GLIC, a prokaryotic ligand-gated ion channel found in Gloeobacter violaceus, served as a model system to comprehend the gating mechanism of eukaryotic ligand-gated channels. The overall architecture of GLIC is similar to the existing structures with each monomer featuring two domains: the ECD, mainly composed of β strands and the TMD, composed of four α helices (M1-M4). In this study, we present cryo-EM structures of GLIC reconstituted in lipid nanodiscs at pH 7.5, 5.5, 4.0, and 2.5. We identified a resting-like state, two putative intermediate states, a putative pre-open state, and an open state.

Two cryo-EM structures of GLIC reconstituted in either soybean polar lipid extract (or asolectin referred to as “aso” onwards) or DOPE:POPS:POPC (2:1:1) at pH 7.5 were obtained with a nominal resolution of 3.4 and 2.9 Å, respectively. Local resolution estimation of these two maps (referred here onwards as GLICaso-pH7.5 and GLICpH7.5) in the apo state shows higher resolution in TMD than ECD. A comparison between GLICaso-pH7.5 and GLICpH7.5 structures shows overlapping secondary structures with minimum conformational differences and a backbone (Cα) RMSD of 0.52 Å. A similar conformation of GLICpH7.5 and GLICaso-pH7.5 confirms the minimal impact of distinct lipid compositions on the GLIC structure in the apo state. Multiple constrictions at the pore of GLICaso-pH7.5 and GLICpH7.5 are observed, with the most significant constrictions at I16´, I9´, and T2´. The highest constriction is observed at I9´ with a radius of ~2.24 Å. However, the radius at I9´ falls below the radius of a hydrated Na+ ion (2.76 Å), reflecting a non-conducting state. Truncated phospholipids (PC in GLICaso-pH7.5 and PE in other structures) were placed in partially resolved non-protein lipid-like densities. In GLICaso-pH7.5, the head group of Lipid 1 is involved in polar interaction with the backbone amide group of M252 located at the M2–M3 loop and this interaction is not observed in GLICpH7.5 and GLICpH5.5. Therefore, our GLICpH7.5 and GLICaso-pH7.5 represent a state closer to the resting conformation.

>[5x]VSPPPPIADEPLTVNTGIYLIECYSLDDKAETFKVNAFLSLSWKDRRLAFDPVRSGVRVKTYEPEAIWIPEIRFVNVENARDADVVDISVSPDGTVQYLERFSARVLSPLDFRRYPFDSQTLHIYLIVRSVDTRNIVLAVDLEKVGKNDDVFLTGWDIESFTAVVKPANFALEDRLESKLDYQLRISRQYFSYIPNIILPMLFILFISWTAFWSTSYEANVTLVVSTLIAHIAFNILVETNLPKTPYMTYTGAIIFMIYLFYFVAVIEVTVQHYLKVESQPARAASITRASRIAFPVVFLLANIILAFLFFGF The widely conserved LytR-CpsA-Psr (LCP) family of enzymes in Gram-positive bacteria is known to attach glycopolymers, including wall teichoic acid, to the cell envelope. In the actinobacterium Actinomyces oris, an LCP homolog here named LcpA is genetically linked to GspA, a glycoprotein that is covalently attached to the bacterial peptidoglycan by the housekeeping sortase SrtA. Further biochemical characterizations provide evidence that LcpA possesses pyrophosphatase activity and also functions as a phosphotransferase, catalyzing glycosylation of the cell wall-anchored protein GspA. Altogether, the findings support that A. oris LcpA is an archetypal LCP enzyme that glycosylates a cell wall-anchored protein, a process that may be conserved in Actinobacteria, given the conservation of LcpA and GspA in these high-GC-content organisms.

The structure of the extracellular LCP domain (eLcpA, residues 78 to 370) was solved at 2.5-Å resolution. Electron density was observed for residues 79 to 106 and 126 to 368, which form a single domain that adopts an α-β-α architecture. A seven‐stranded antiparallel β‐sheet forms the core of the protein with a total of eight α‐helices flanking the β-sheet on both of its faces, forming a hydrophobic tunnel. The tunnel is ∼23 Å in length and is lined by residues located on the central β-sheet and helices H5, H6, and H7. The surface of the tunnel contains many nonpolar residues consistent with it interacting with lipid substrates. Interestingly, during refinement additional electron density was observed near the exit point of the tunnel, defined by helices H6 and H7, indicating that a ligand was bound. The best match to the data was obtained by modeling the ligand as a PEG 4000 molecule that was used as a precipitant during crystallization. This ligand is bound with 50% occupancy and defines the exit point for the tunnel distal to the active site. In A. oris LcpA, R128, R149, and R266 are conserved residues, which cluster together within a surface-exposed pocket (shown in red). Intriguingly, unlike other LCP enzymes, LcpA contains a disulfide bond, formed between residues C179 and C365, linking the C terminus to α-helix H2.

> AHRPARVDIAMPTTSSPTAGETWLILGTDSRATVPGDQNRYGTTQEVEGSRADVIALVRPSQEGVTIINLPRDLTINSKGMELDRLATTYVPGPQNTVNALCTGLGIPTTHLVTIDMAQFATIIDSLGGIEVDVPEPVRDAYTGLNLSSAGRHRLSGIDALALVRSRHPEILRDGRWVTMSQADGAQRRSQSTATVMQAVLSAIGQKASNPVSLHQLAHTVAGNITLDSGTGLSDLAALGRSASKARRAGATTIIDLPTGPRDESIIVSPNQESRDLLARYGYSPKTCRPAGA N-{(2R)-2-methyl-3-[4-(propan-2-yl)phenyl]propanoyl}-beta-D-glucopyranosylamine | C19 H29 N 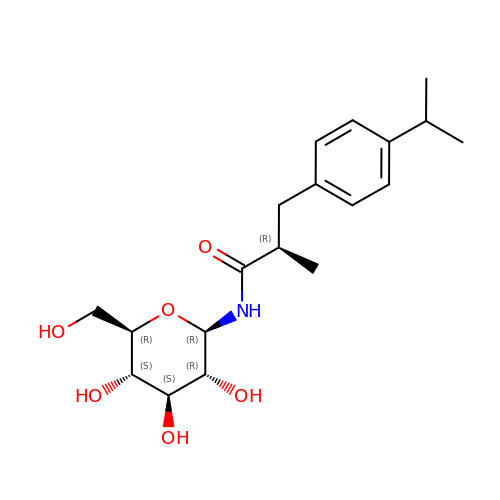O6 | HJOFLVJJICDECE-YMZRVSMESA-N>[4x]MIPGKPWDTPQLAAELERWKLDGRDVSLLIG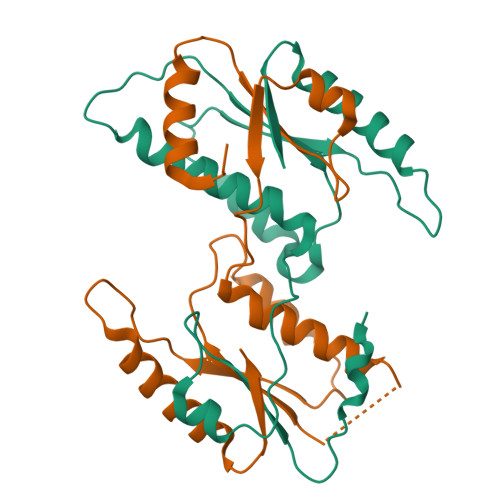GPEGLSPACKAAAEQSFSLSALTLPHPLVRVLVAESLYRAWSITTNHPYHREGSMKLQLVAVGTKMPDWVQTGFTEYLRRFPKDMPFELIEIPAGKRGKNADIKRILDKEGEQMLAAAGKNRIVTLD> MDTSSKENIQLFCKTSVQPVGRPSFKTEYPSSEEKQPCCGELKVFLCALSFVYFAKALAEGYLKSTITQIERRFDIPSSLVGVIDGSFEIGNLLVITFVSYFGAKLHRPKIIGAGCVIMGVGTLLIAMPQFFMEQYKYERYSPSSNSTLSISPCLLESSSQLPVSVMEKSKSKISNECEVDTSSSMWIYVFLGNLLRGIGETPIQPLGIAYLDDFASEDNAAFYIGCVQTVAIIGPIFGALLGSLCAKLYVDIGFVNLDHITITPKDPQWVGAWWLGYLIAGIISLLAAVPFWYLPKSLPRSQSREDSNSSSEKSKFIIDDHTDYQTPQGENAKIMEMARDFLPSLKNLFGNPVYFLYLCTSTVQFNSLFGMVTYKPKYIEQQYGQSSSRANFVIGLINIPAVALGIFSGGIVMKKFRISVCGAAKLYLGSSVFGYLLFLSLFALGCENSDVAGLTVSYQGTKPVSYHERALFSDCNSRCKCSETKWEPMCGENGITYVSACLAGCQTSNRSGKNIIFYNCTCVGIAASKSGNSSGIVGRCQKDNGCPQMFLYFLVISVITSYTLSLGGIPGYILLLRCIKPQLKSFALGIYTLAIRVLAGIPAPVYFGVLIDTSCLKWGFKRCGSRGSCRLYDSNVFR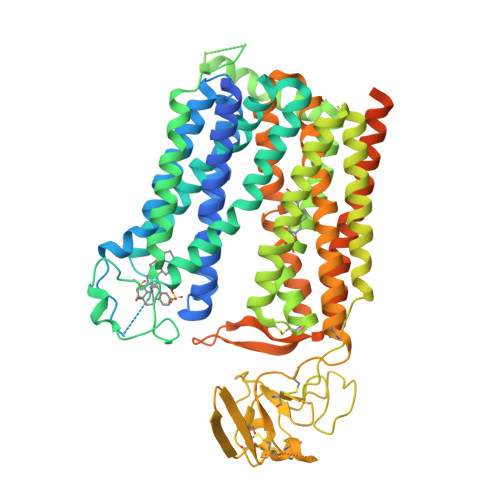HIYLGLTVILGTVSILLSIAVLFILKKNYVSKHRSFITKRERTMVSTRFQKENYTTSDHLLQPNYWPGKETQLAAALEVLFQGPGAAEDQVDPRLIDGKHHHHHHHH> MASLPKRIIKETEKLVSDPVPGITAEPHDDNLRYFQVTIEGPEQSPYEDGIFELELYLPDDYPMEAPK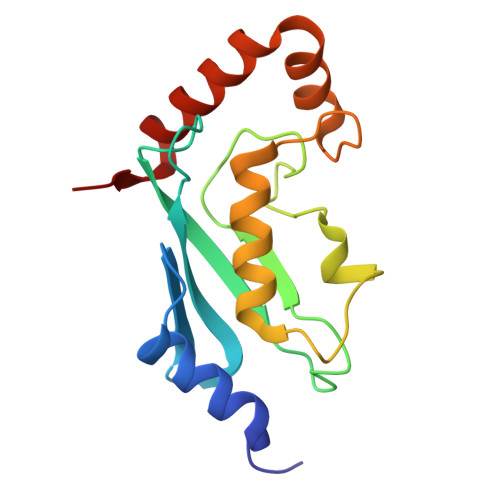VRFLTKIYHPNIDRLGRICLDVLKTNWSPALQIRTVLLSIQALLASPNPNDPLANDVAEDWIKNEQGAKAKAREWTKLYAKKKP>[3x]GSHMEAVQNRIVEAAERVPGVRGVIHLRARYVGQDIWADMIIGVDPENTVEQAHEICE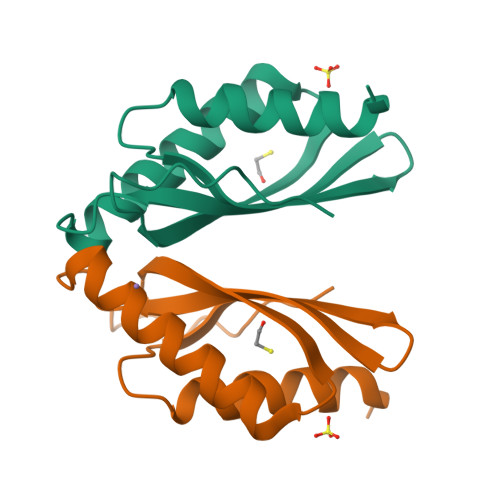AVQAAVCGKIRRIESLHVSADAREIGDTTKPSFSDQPLSFDEVMLSKVDN> MAPIAYGVYSQADGVSPYLKVTLTNSQYQVTGYISQGAAMNMAQNWEAPFTGMSMGSVSGALGGFVQVGTETTSVA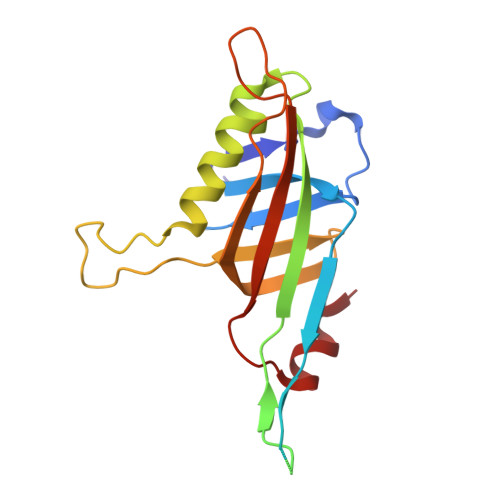RWNSLMVWEGGTPPTFTLPVTFIALNNPFIEVSGAIAALTAMISPELKAANVGGQIPERVTLNIGRRINITDVAIQDLSFDLDAPRDSNGYFLKNTVNLQLTGSSIYNSSDIVRAFQ>MAHHHHHHSLNQINIEIAYAFPERYYLKSFQVDEGITVQTAITQSGILSQFPEIDLSTNKIGIFSRPIKLTDVLKEGDRIEIYRPL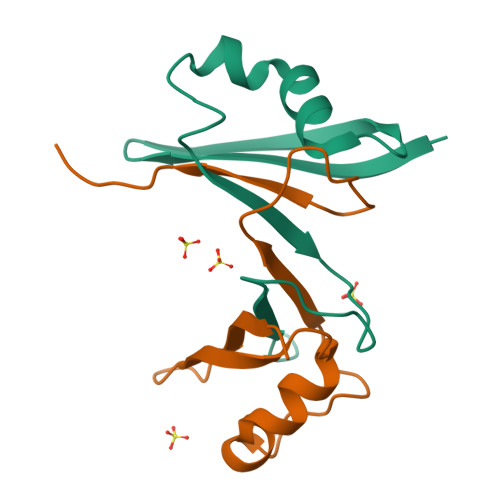LADPKEIRREG[2x]>[2x]MSALFEPYTLKDVTLRNRIAIPPMCQYMAEDGMINDWHHVHLAGLARGGAGLLVVEATAVAPEGRITPGCAGIWSDAHAQAFVPVVQAIKAAGSVPGIQIAHAGRKASANRPWEGDDHIAADDTRGWETIAPSAIAFGAHLPKVPREMTLDD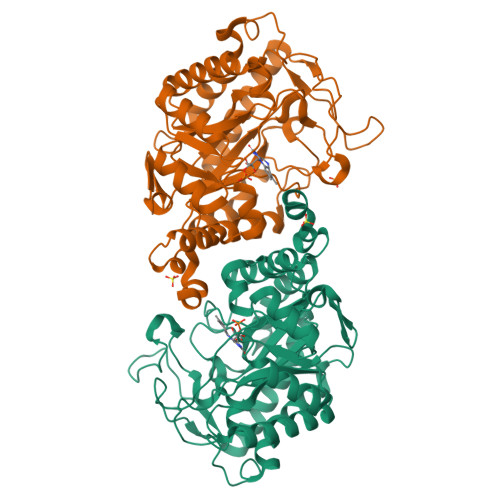IARVKQDFVDAARRARDAGFEWIELHFAHGYLGQSFFSEHSNKRTDAYGGSFDNRSRFLLETLAAVREVWPENLPLTARFGVLEYDGRDEQTLEESIELARRFKAGGLDLLSVSVGFTIPDTNIPWGPAFMGPIAERVRREAKLPVTSAWGFGTPQLAEAALQANQLDLVSVGRAHLADPHWAYFAAKELGVEKASWTLPAPYAHWLERYR>GSITVAVLQDGSIIPVEELPLEKAPVVNILRVPFTEGLFLVSNRGRVYWIAGSQALQGSKVSLKSREEKIVGAFIREKFGNRLLLATKKGYVKKIPLAEFEYKAQGMPIIKLTEGDEVVSIASSVDETHILLFTKKGRVARFSVREVP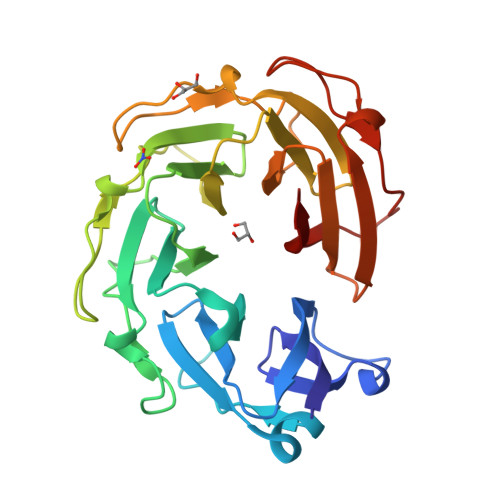PSTPGARGVQGIKLEKNDETSGLRIWNGEPYLLVITAKGRVKKISHEEIPKTNRGVKGTEVSGTKDTLVDLIPIKEEVELLITTKNGKAFYDKINQKDIPLSTKKSIPRTRWKLEDDEIIKVVIKKSE[3x]> MPEQYRYTLPVKAGEQRLLGELTGAACATLVAEIAERHAGPVVLIAPDM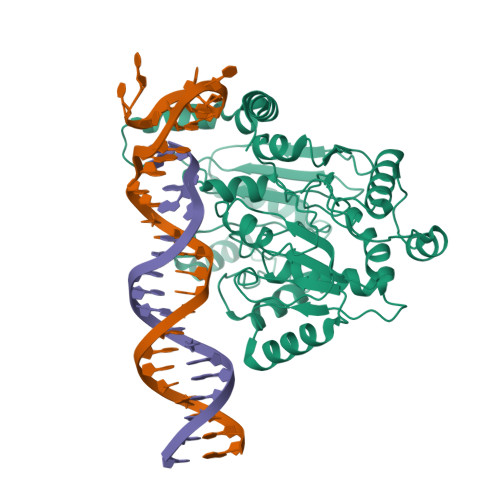QNALRLHDEISQFTDQMVMNLADWETLPYDSFSPHQDIISSRLSTLYQLPTMQRGVLIVPVNTLMQRVCPHSFLHGHALVMKKGQRLSRDALRTQLDSAGYRHVDQVMEHGEYATRGALLDLFPMGSELPYRLDFFDDEIDSLRVFDVDSQRTLEEVEAINLLPAHEFPTDKAAIELFRSQWRDTFEVKRDPEHIYQQVSKGTLPAGIEYWQPLFFSEPLPPLFSYFPANTLLVNTGDLETSAERFQADTLARFENRGVDPMRPLLPPQSLWLRVDELFSELKNWPRVQLKTEHLPTKAANANLGFQKLPDLAVQAQQKAPLDALRKFLETFDGPVVFSVESEGRREALGELLARIKIAPQRIMRLDEASDRGRYLMIGAAEHGFVDTVRNLALICESDLLGERVARRRQDSRRTINPDTLIRNLAELHIGQPVVHLEHGVGRYAGMTTLEAGGITGEYLMLTYANDAKLYVPVSSLHLISRYAGGAEENAPLHKLGGDAWSRARQKAAEKVRDVAAELLDIYAQRAAKEGFAFKHDREQYQLFCDSFPFETTPDQAQAINAVLSDMCQPLAMDRLVCGDVGFGKTEVAMRAAFLAVDNHKQVAVLVPTTLLAQQHYDNFRDRFANWPVRIEMISRFRSAKEQTQILAEVAEGKIDILIGTHKLLQSDVKFKDLGLLIVDEEHRFGVRHKERIKAMRANVDILTLTATPIPRTLNMAMSGMRDLSIIATPPARRLAVKTFVREYDSMVVREAILREILRGGQVYYLYNDVENIQKAAERLAELVPEARIAIGHGQMRERELERVMNDFHHQRFNVLVCTTIIETGIDIPTANTIIIERADHFGLAQLHQLRGRVGRSHHQAYAWLLTPHPKAMTTDAQKRLEAIASLEDLGAGFALATHDLEIRGAGELLGEEQSGSMETIGFSLYMELLENAVDALKAGREPSLEDLTSQQTEVELRMPSLLPDDFIPDVNTRLSFYKRIASAKTENELEEIKVELIDRFGLLPDPARTLLDIARLRQQAQKLGIRKLEGNEKGGVIEFAEKNHVNPAWLIGLLQKQPQHYRLDGPTRLKFIQDLSERKTRIEWVRQFMRELEENAIA The HCV NS3/4A protease – a chymotrypsin-like serine protease – is a prime therapeutic target that cleaves four known sites along the virally encoded polyprotein. The NS3/4A protease also hydrolyzes two human proteins, TRIF and MAVS, which are part of the innate immune system, thereby confounding the innate immune response to viral infection. In this study, we report that four chemically representative protease inhibitors – telaprevir, danoprevir, vaniprevir and MK-5172 – exhibit distinct susceptibilities to the protease variants R155K, A156T and D168A. To elucidate the underlying mechanism by which chemically diverse inhibitors bind to the wild-type protease and drug-resistant variants, crystal structures were determined for 16 inhibitor-protease complexes. These complexes include wild-type protease and resistant variants R155K, D168A and A156T each bound to telaprevir, danoprevir, vaniprevir and MK-5172, with resolutions ranging from 1.10–2.50 Å; S139A protease variants were used except for telaprevir, which requires covalent bond formation with the serine 139 for efficient binding.

However, the A156T mutation resulted in a steric clash with telaprevir's P2 moiety, causing the inhibitor to shift significantly; the inhibitor P2 moiety moved away from R155, losing van der Waals interactions with the protease. Notably, in the A156T-telaprevir complex the covalent bond between the ketoamide warhead and the catalytic serine was extended to greater than 2 Å, suggesting a reduced capacity for covalent modification, consistent with the large loss in potency against A156T. Thus, while telaprevir's flexibility allows adaptation to D168A, it cannot accommodate the disruption by R155K or A156T. Telaprevir and other linear ketoamide drugs select for A156T variants by direct steric clashes, while linear (BI 201335) and macrocyclic drugs (danoprevir, vaniprevir, TMC435) with large P2 moieties select for D168A variants by disrupting favorable stacking interactions with R155.

> GSHMASMKKKGSVVIVGRINLSGDTAYAQQTRGEEGCQETSQTGRDKNQVEGEVQIVSTATQTFLATSINGVLWTVYHGAGTRTIASPKGPVTQMYTNVDKDLVGWQAPQGSRSLTPCTCGSSDLYLVTRHADVIPVRRRGDSRGSLLSPRPISYLKGSSGGPLLCPAGHAVGIFRTAVSTRGVAKAVDFIPVESLETTMRSP> GQSIMTVRTTHTEVEVHAGGTVELPCSYQLANDTQPPVISWLKGASPDRSTKVF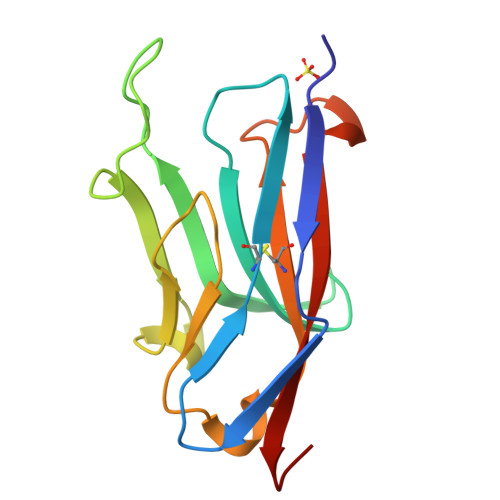KGNYNWQGEGLGFVESDSYKESFGDFLGRASVANLAAPTLRLTHVHPQDGGRYWCQVAQWSIRTEFGLDAKSVVLKVTGHT> GSHMQQPEGVTAPGNEPMAIPSDYKLVWADEFNTPGAPDAKKWRYDTSRNKEGWYNNELQYYAAGRPENVRVENGNLVIETRKERLTSMADYGGQEYSSGKLFTQGLADWQYGYVEVRAKLACGKGMWPAIWMMASDGSTGWPALGSIDIMEMVAWDPTTIHGTIHTKAYNHVIHTQKGSRTTAADPCGQFHTYSLDWTKDRMLIGVD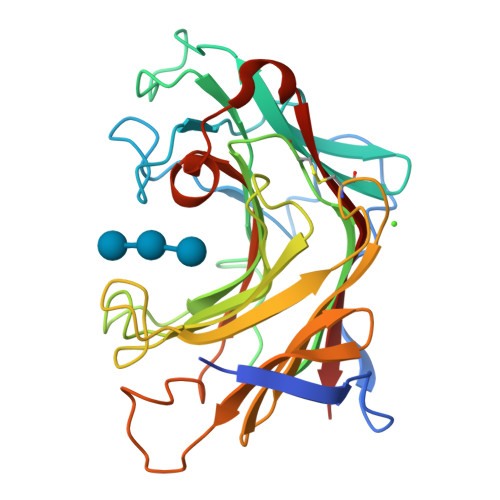GHAYMRFDNDHKGNHDTWPFDSPQYLILNVAIGGWGGQQGVDAAAFPSKMEVDYVRVYQKR> GPVPTPPDNIQVQENFNISRIYGKWYNLAIGSTSPWLKKIMDRMTVSTLVLGEGATEAEISMTSTRWRKGVCEETSGAYEKTDTDGKFLYHKSK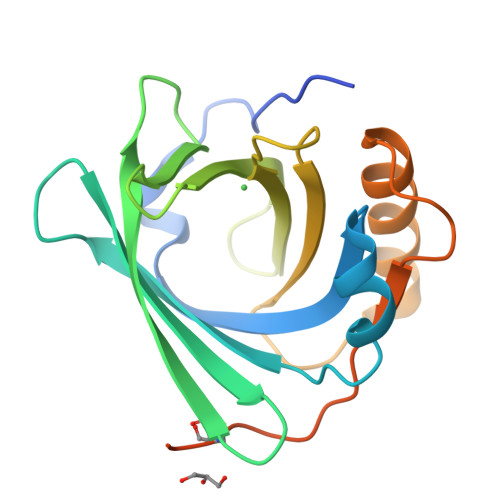WNITMESYVVHTNYDEYAIFLTKKFSRHHGPTITAKLYGRAPQLRETLLQDFRVVAQGVGIPEDSIFTMADRGECVPGEQEPEPILIPRSAWSHPQFEK>SIKTPEDIEKMRVAGRLAAEVLEMIEPYVKPGVSTGELDRICNDYIVNEQHAVSACLGYHGYPKSVCISINEVVCHGIPD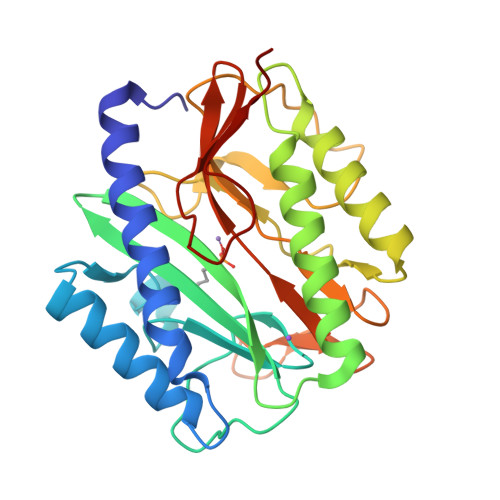DAKLLKDGDIVNIDVTVIKDGFHGDTSKMFIVGKPTIMGERLCRITQESLYLALRMVKPGINLREIGAAIQKFVEAEGFSVVREYCGHGIGRGFHEEPQVLHYDSRETNVVLKPGMTFTIEPMVNAGKKEIRTMKDGWTVKTKDRSLSAQYEHTIVVTDNGCEILTLRKDDTIPAIISHDE[2x]> MNLPTAQEVQGLMARYIELVDVGDIEA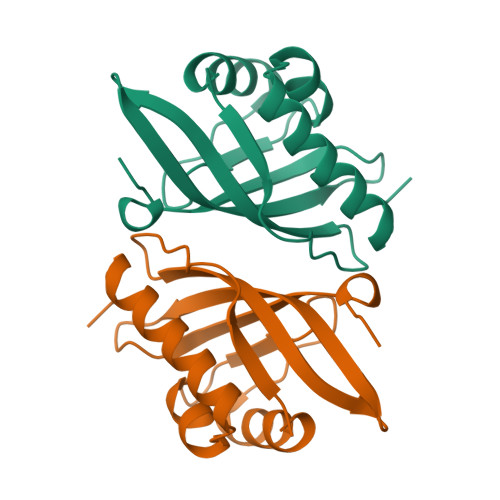IVQMYADDATVEDPFGQPPIHGREQIAAFYRQGLGGGKVRACLTGPVRASHNGCGAMPFRVEMVWNGQPCALDVIDVMRFDEHGRIQTMQAYWSEVNLSVREPQ> MNRIPALR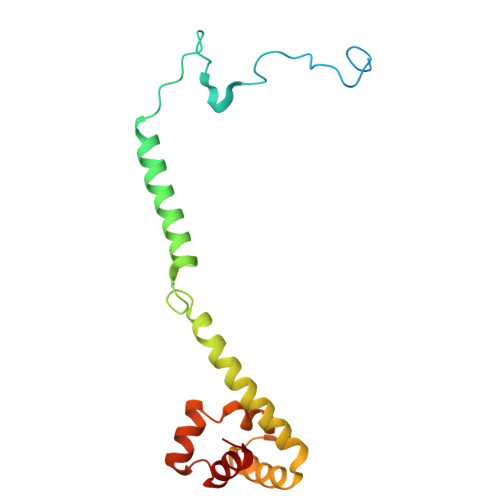RIGAQALRNPVTRAGGASGHPNGSFWSEGTQVGLNGFKYGEIPLPNGQPRKKLWLENIWNIGYGGFFLGAFCLYYGAPPGHVIPSQWATPKAKDEYAVDMKMIDKYNERPDLQARLSIVLKDLNMIEEEAYDLIMMRKDYKVLLGLHSGRVPADLKAIYEELEA> MASARGY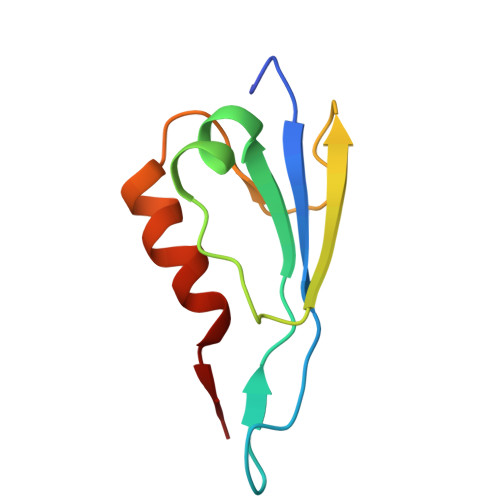VNIKTFEQKLDGNKKIEGKEVSVAFPLYSDVHKISGAHYQTFPSEKAAYSTVYEENQRTEWIAANEDLWKVTG> GS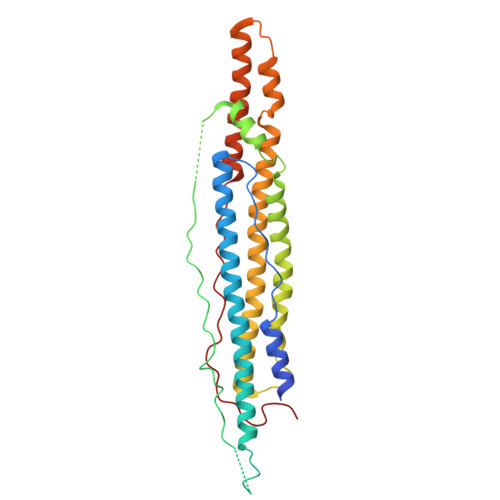MSEELQYELPGLERKAHECESTRPEGPGDATKPDELATTASVYSKLMASAAKLKATFAAGDREGERIAAAIRAAAGAYQKIEEQKAAELSRQMNGSDAPPPAAEAVVPDMSGIPGPLAIPSMEYPSAAAAADEMDWEAAARIIHSGDTQALSMKYFRDQWRDYQSTLEGHGRHFANPAEGWAGAAAETCAEAQRRLSTWWADMGAECGRLAQEATTFVDAHDKLVANHPTLENVREFEETEWASEWDRQNAWAMLQEQSEDALEAYANGSQIQEIRPGKPPSIGGLPAVNDGDVQA>AALPDQSFLWNVFQRVDKDRSGVISDTELQQAL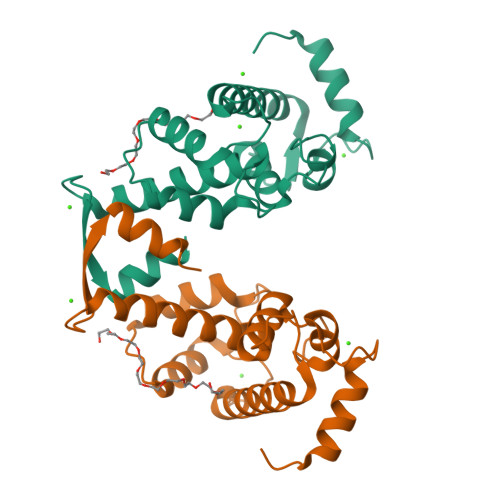SNGTWTPFNPVTVRSIISMFDRENKAGVNFSEFTGVWKYITDWQNVFRTYDRDNSGMIDKNELKQALSGFGYRLSDQFHDILIRKFDRQGRGQIAFDDFIQGCIVLQRLTDIFRRYDTDQDGWIQVSYEQYLSMVFSIV[2x]> MKPLYRQLKSSHYSSDYSSPGYLAAEAVYAEIGYELDTLLKQNPGYANTCAVRMSLALLKTGISFKGRLPIKKGAYKG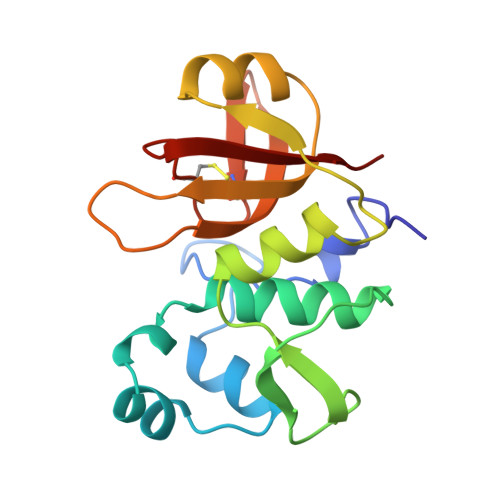KTIEPGAKLLADQLHRSSSFGKAKIFFNAPDAEKGIGNKKGVVFFNKITNYDGGHIDLIEPENSLLTCHSHCYFNCKEVWFWELS(3~{S},6~{S})-3-[(4-hydroxyphenyl)methyl]-6-[(2-methyl-4-oxidanyl-phenyl)methyl]piperazine-2,5-dione | C19 H20 N2 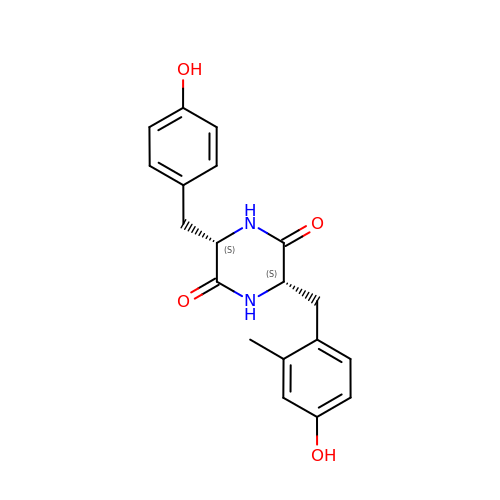O4 | OLLRPTQZHVLIEA-IRXDYDNUSA-N>AMITPPGAGVKDKKRAILEATLAVLRERGLSGLKMEEVARRAEVGKGTIYLYFRDKRDLLKALVEERTWAFYREVEEVVRRKAPFFVRLEEVLRRRLAWVQEWRGLWAAVAREAMDDPTPW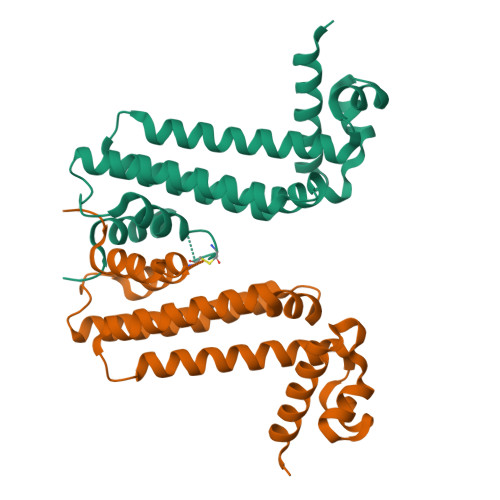LKGLHEHYLRLLEELLRSGQSEGAVRTGLSPRATAAVIAAMGCTPSLEVEAYLEHLMEVLRKGVEP[4x]> GAMESKKRQWALEDFEIGRPLGKGKFGNVYLAREKQSKFILALKVLFKAQLEKAGVEHQLRREVEIQSHLRHPNILRLYGYFHDATRVYLILEYAPLGTVYRELQKLSKFDEQRTATYITELANALSYCHSKRVIHRDIKPENLLLGSAGELKIADFGWSVHAPSSRRTTLAGTLDYLPPEMIEGRMHDEKVDLWSLGVLCYEFLVGKPPFEANTYQETYKRISRVEFTFPDFVTEGARDLISRLL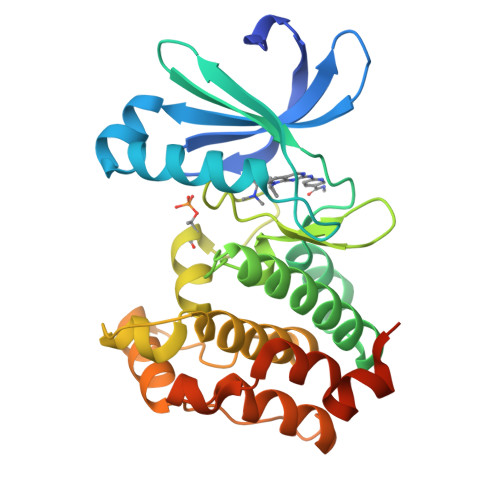KHNPSQRPMLREVLEHPWITANSSKPSNSQNKESASKQS> MATVAVEETGACLLCYTIHFVLKCIAVARVGDVLLTCAGTRSLWRTLSPLRHSLSPLFLSLSLSLFPALPGNCAYGSRVKTSAFSLTLPAERCRRVLEEGREAQGTTVAVNRTLAPSLLLPTANTNLCTPRGTLVEAMLRPTCALAAAEFKQKSRWSSVWPNMRYGSMYLNYSVGRQLPMKGVNWVTRDSNRLTNFAARYSSVIEDVDVKRNEEELNIQMSDVRWNDHRRIYWKCSFCGSSYRKNVSVRTKYHAGCNFCKGRYASEVLREQTPVVALREAQPELFKGLAENEKNDNIGSLSVTSKFRAEWKCQSCGQPYRATIRSRTGLTEPGQAPLHPRITEWSAHCPACAWRTNMTAIGRKAQEEGQYLGLETSLAELTGAAAGKRIP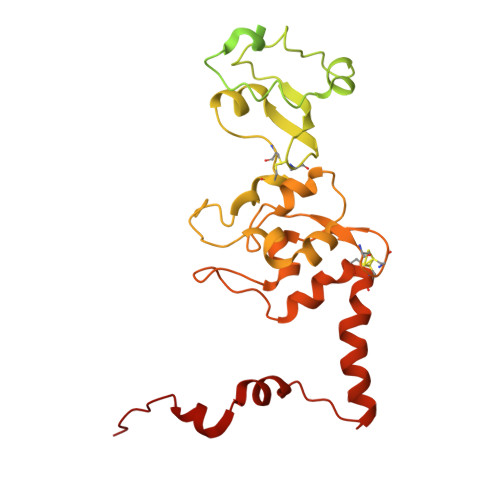RRRKLVA>[4x]IVGGYTCEENSLPYQVSLNSGSHFCGG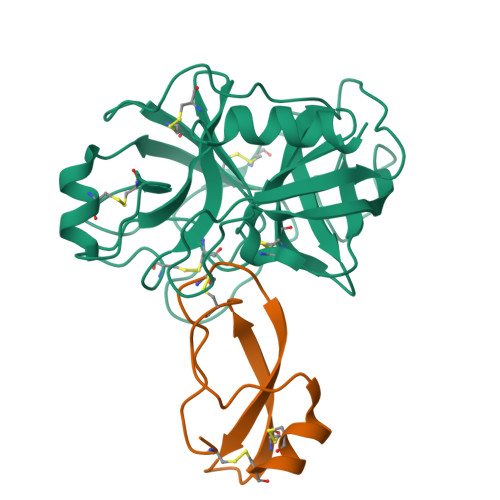SLISEQWVVSAAHCYKTRIQVRLGEHNIKVLEGNEQFINAAKIIRHPKYNRDTLDNDIMLIKLSSPAVINARVSTISLPTAPPAAGTECLISGWGNTLSFGADYPDELKCLDAPVLTQAECKASYPGKITNSMFCVGFLEGGKDSCQRDAGGPVVCNGQLQGVVSWGHGCAWKNRPGVYTKVYNYVDWIKDTIAANS;>VCSEQAETGPCRAMISRWYFDVTEGKCAPFFYGGCGGNRNNFDTEEYCMAVC[4x]> HHHHHHMPIQVLPPQLANQIAAGEVVERPASVVKELVENSL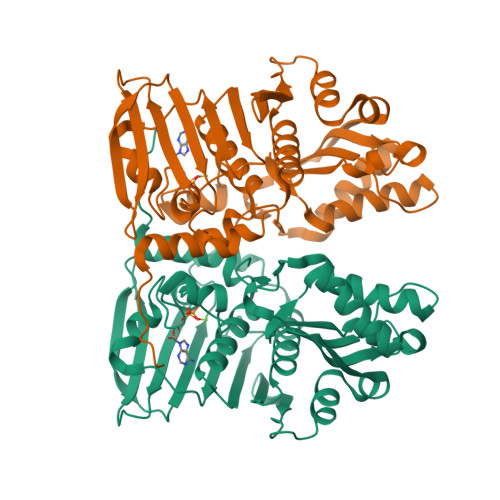DAGATRIDIDIERGGAKLIRIRDNGCGIKKDELALALARHATSKIASLDDLEAIISLGFRGEALASISSVSRLTLTSRTAEQQEAWQAYAEGRDMNVTVKPAAHPVGTTLEVLDLFYNTPARRKFLRTEKTEFNHIDEIIRRIALARFDVTINLSHNGKIVRQYRAVPEGGQKERRLGAICGTAFLEQALAIEWQHGDLTLRGWVADPNHTTPALAEIQYCYVNGRMMRDRLINHAIRQACEDKLGADQQPAFVLYLEIDPHQVDVNVHPAKHEVRFHQSRLVHDFIYQGVLSVLQQQLETPLPLDDEPQPAPR The bifunctional enzyme proline utilization A (PutA) catalyzes the two-step oxidation of L-proline to L-glutamate using proline dehydrogenase (PRODH) and L-glutamate-γ-semialdehyde dehydrogenase (GSALDH) domains. The two active sites are 42 Å apart and connected by a buried tunnel that is hypothesized to channel the intermediates Δ1-pyrroline-5-carboxylate (P5C) and/or L-glutamate-γ-semialdehyde (GSAL). The PRODH active site is located in a (βα)8 barrel, while the GSALDH module features Rossmann NAD+-binding and catalytic domains, which are both characteristic of the ALDH superfamily. Kinetic and conventional X-ray crystallography of PutA from Sinorhizobium meliloti (SmPutA) were used to capture high resolution (1.47–1.88 Å) structures of states along the catalytic cycle, including a novel FADH−-proline covalent adduct in the PRODH site, the intermediate P5C bound noncovalently in the reduced PRODH active site, the covalent acyl-enzyme intermediate of the GSALDH reaction, and noncovalent complexes of GSAL and the final product L-glutamate in the GSALDH active site.

The structure of the acyl-enzyme intermediate was captured by soaking crystals of the E810A variant in 40 mM L-proline, 1 mM Coenzyme Q1, and 1 mM NAD+ for 24 h and then flash-cooling the crystal in liquid nitrogen. Glu810 is the conserved glutamate in the GSALDH active site that facilitates hydrolysis of the acyl-enzyme intermediate, and mutation to Ala is expected to slow the hydrolysis step, allowing the acyl-enzyme intermediate to build up. The structure of the acyl-enzyme intermediate was resolved at 1.74 Å resolution. Electron density clearly showed the presence of a covalent modification of Cys844 in chain A. The electron density is consistent with the acyl-enzyme intermediate, which was modeled with occupancy of 0.83. The covalently bound GSAL is stabilized by the same interactions described above for noncovalent GSAL, involving the oxyanion hole, aromatic box, and anchor loop. Electron density for the coenzyme, either NAD+ or NADH, was also observed (occupancy of 1.0 in both chains). The coenzyme adopts the pose associated with NAD+ prior to hydride transfer (hydride transfer pose) and is distinct from the pose associated with NADH in which the nicotinamide riboside has withdrawn from the catalytic pocket. Given that the coenzyme is in the pose typical for NAD+, we have modeled it as NAD+. Interestingly, the ion pair gate is open in the noncovalent GSAL complex and closed in the acyl-enzyme.

>[2x]SMMSPNPLQKPAIDAAPAPFADFAPPVRPQSTLRRAITAAYRRPETECLPPLVEAATQSKEIRDAAASTARKLIEALRGKHSGSGVEGLVQEYSLSSQEGVALMCLAEALLRIPDTATRDALIRDKIADGNWKSHLGGSRSLFVNAATWGLVVTGKLTSTVNDRSLAAALTRLISRCGEPVIRRGVDMAMRMMGEQFVTGETIREALKRSKELEEKGFSYSYDMLGEAATTAADAERYYRDYESAIHAIGKASAGRGIYEGPGISIKLSALHPRYSRAQAARVMGELLPRVKALALLAKNYDIGLNIDAEEADRLELSLDLLEVLCLDGDLSGWNGMGFVVQAYGKRCPFVLDFIIDLARRSGRRIMVRLVKGAYWDAEIKRAQLDGLADFPVFTRKIHTDVSYIACAAKLLAATDVVFPQFATHNAQTLAAIYHMAGKDFHVGKYEFQCLHGMGEPLYEEVVGRGKLDRPCRIYAPVGTHETLLAYLVRRLLENGANSSFVHRINDPKVSIDELIADPVEVVRAMPVVGAKHDRIALPAELFGDARTNSAGLDLSNEETLASLTEALRESAAMKWTALPQLATGPAAGETRTVLNPGDHRDVVGSVTETSEEDARRAVRLAADAAPDWAAVPPSERAACLDRAAELMQARMPTLLGLIIREAGKSALNAIAEVREAIDFLRYYAEQTRRTLGPGHGPLGPIVCISPWNFPLAIFTGQIAAALVAGNPVLAKPAEETPLIAAEGVRILREAGIPASALQLLPGDGRVGAALVAAAETAGVMFTGSTEVARLIQAQLADRLSPAGRPIPLIAATGGQNAMIVDSSALAEQVVGDVITSAFDSAGQRCSALRVLCLQEDVADRILTMLKGALHELHIGRTDRLSVDVGPVITSEAKDNIEKHIERMRGLGRKVEQIGLASETGVGTFVPPTIIELEKLSDLQREVFGPVLHVIRYRRDDLDRLVDDVNATGYGLTFGLHTRLDETIAHVTSRIKAGNLYINRNIIGAVVGVQPFGGRGLSGTGPKAGGPLYLGRLVTTAPVPPQHSSVHTDPVLLDFAKWLDGKGARAEAEAARNAGSSSALGLDLELPGPVGERNLYTLHARGRILLVPATESGLYHQLAAALATGNSVAIDAASGLQASLKNLPQTVGLRVSWSKDWAADGPFAGALVEGDAERIRAVNKAIAALPGPLLLVQAASSGEIARNPDAYCLNWLVEEVSASINTAAAGGNASLMAIG The Vtc4p β-tunnel domain is not unique to eukaryotic polyP polymerases but is a structural hallmark of triphosphate tunnel metalloenzymes (TTMs), whose characteristic features are the presence of a topologically closed hydrophilic β-barrel, the preference for triphosphate-containing substrates, and for a divalent metal co-factor (PFAM families CYTH and VTC). Members of the ancient triphosphate tunnel metalloenzyme family can be found in all kingdoms of life. Our comparative analysis defines that most of these enzymes share a common catalytic mechanism in their tunnel centers, yet they have evolved different substrate recognition modes on their tunnel entries. The observed substrate plasticity apparently allows TTM proteins to act on a wide array of enzyme substrates and to perform very different reactions, many of which likely remain to be discovered.

To assess the functional relevance of the observed metal co-factors in AtTTM3, we studied substrate binding and metal ion coordination in the evolutionary distant TTM ygiF from E. coli. YgiF shares ∼18% sequence identity with AtTTM3 and has the same catalytic activity and substrate specificity. The structure of full-length ygiF was solved using iodide/sulfur SAD phasing and reveals the conserved TTM fold (r.m.s.d. with the AtTTM3 tunnel domain is 2.0 Å compared with 172 corresponding Cα atoms, and 0.65 Å comparing 75 corresponding Cα in the tunnel center). ygiF contains a second, α-helical domain, which is connected to the TTM by a well ordered linker (residues 201–221, cyan in Fig. 3C) and which has been previously annotated as CHAD domain. We next solved structures of ygiF in complex with PPPi and in the presence of either MgCl2 or MnCl2. The ygiF triphosphate substrate is bound in the same conformation as observed in AtTTM3, and we could identify two metal co-factors. One Mg2+/Mn2+ ion is again found coordinated by tripolyphosphate and by Glu-160ygiF, which corresponds to Glu-169 in AtTTM3 (position 1 in Fig. 3D). The second Mg2+/Mn2+ ion is coordinated by three glutamate residues from the acidic patch in ygiF (Glu-4ygiF, Glu-6ygiF, Glu-162ygiF) and by a water molecule that is positioned close to a terminal phosphate of the tripolyphosphate substrate (position 2). Taken together, our experiments define two consistent Mg2+/Mn2+ coordination centers in plant and bacterial TTM tripolyphosphatases. Consistently, changing the corresponding Glu-6ygiF and Glu-160ygiF to Ala impairs the enzymatic activity of ygiF, suggesting that the proper arrangement of metal binding sites 1 and 2 in the tunnel center is essential for catalysis.

> GAMAQEIELKFIVNHSAVEALRDHLNTLGGEHHDPVQLLNIYYETPDNWLRGHDMGLRIRGENGRYEMTMKVAGRVTGGLHQRPEYNVALSEPTLDLAQLPTEVWPNGELPADLASRVQPLFSTDFYREKWLVAVDDSRIEIALDQGEVKAGEFAEPICELELELLSGDTRAVLKLANQLVSQTGLRQGSLSKAARGYHLAQGNPAREIKPTTILHVAAKADVEQGLEAAFELALAQWQYHEELWVRGNDAAKEQVLAAIGLVRHALMLFGGIVPRKASTHLRDLLTQCEATIASAVSAVTAVYSTETAMAKLALTEWLVSKAWQPFLDAKAQGKISDSFKRFADIHLSRHAAELKSVFCQPLGDRYHDQLPRLTRDIDSILLLAGYYDPVVAQAWLENWQGLRHAIATGQRIEIEHFRNEANNQEPFWLHSGKR> MLKRLQVKNFRCLEDIDLPLGPLTAIVGPNGAGKTTILRAIDLVLGDVWPSLRSFRIPQDFINFDTTRAIEITVHFDPPYTQGSFNITAFRLTCKGEDADFHVDLEPLDEGGNVPRYPSGNPLRVGTDMRNHARVLFLDHRRNLAQHLPSIRGSILGRLLQPVRREFKLQDNFKQVYEQAMDLLRTEQVKQIEKTIAETAKQMLGFLGKDAMKSMEIGFGFADPANPFNSLRLQYRESDLTLPGDELGLGIQSAIVVGIFEAFRQLGEKIGTVIIEEPEMYLHPQ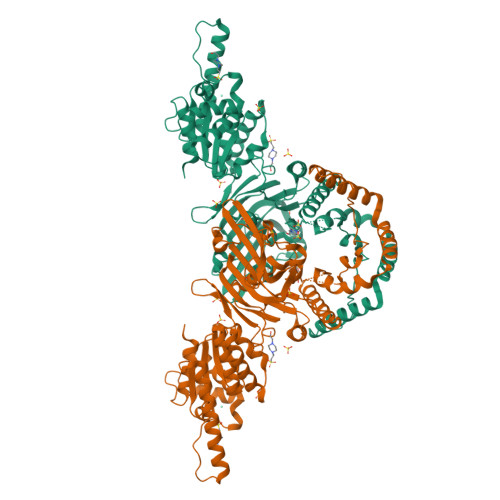AQRYFYRLLCEMADKDQCQIIYSTHSPIFADVNRFEALRLVRKDRDDRVVVSYVREEDKSALDNVRNRFKLGGRFDTARNEVLFAKRALLVEGYGDRVAALQLFNQLEVDPDAECIAVVDCGGKAGIELIVGVCKALDIPFVVVHDEDVWPIDERADEETRRKQEQENKAEQEKNQRIQACAGAERVFVVQPSLEAALGIGRNASDKPYRIAEILKTVDVGQPPDALRPFVEAIRQVTRPMEE>MASLRSRCDQLEERVSAAEDEINEIKREGKFREKRIKRNEQSLQEIWDYVKRPNLRLIGVPESDVENGTKLENTLQDIIQENFPNLARQANVQIQEIQRTPQRYSSRRATPRHIIVRFTKVEMKEKMLRAAR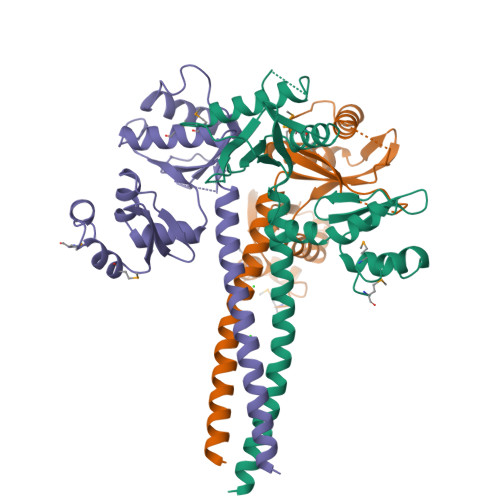EKGRVTLKGKPIRLTVDLSAETLQARREWGPIFNILKEKNFQPRISYPAKLSFISEGEIKYFIDKQMLRDFVTTRPALKELLKEALNMERNNRYQHHHHHH[3x]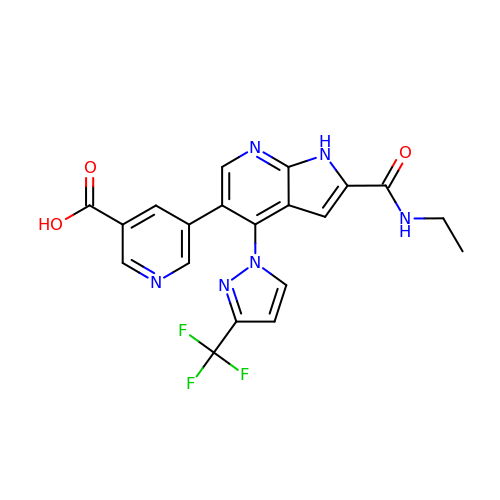5-{2-(ethylcarbamoyl)-4-[3-(trifluoromethyl)-1H-pyrazol-1-yl]-1H-pyrrolo[2,3-b]pyridin-5-yl}pyridine-3-carboxylic acid | C20 H15 F3 N6 O3 | QEODWPGJXCSBCR-UHFFFAOYSA-N> HGSPVDICTAKPRDIPMNPMCIYRSPEKKATEDEGSEQKIPEATNRRVWELSKANSRFATTFYQHLADSKNDNDNIFLSPLSISTAFAMTKLGACNDTLQQLMEVFKFDTISEKTSDQIHFFFAKLNCRLYRKAAKSSKLVSANRLFGDKSLTFNETYQDISELVYGAKLQPLDFKENAEQSRAAINKWVSNKTEGRITDVIPSEAINELTVLVLVNTIYFKGLWKSKFSPENTRKELFYKADGESCSASMMYQEGKFRYRRVAEGTQVLELPFKGDDITMVLILPKPEKSLAKVEKELTPEVLQEWLDELEEMMLVVHMPR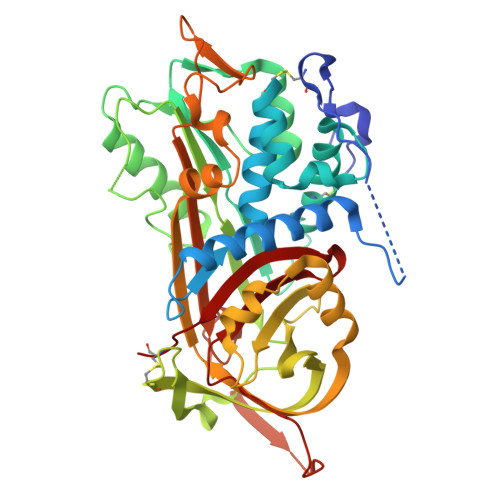FRIEDGFSLKEQLQDMGLVDLFSPEKSKLPGIVAEGRDDLYVSDAFHKAFLEVNEEGAEAAASTAVVIAGRSLNPNRVTFKANRPFLVFIREVPLNTIIFMGRVANPCVK N-(8-methyl-2-phenylimidazo[1,2-a]pyrazin-3-yl)-2-(10H-phenoxazin-10-yl)acetamide | C27 H21 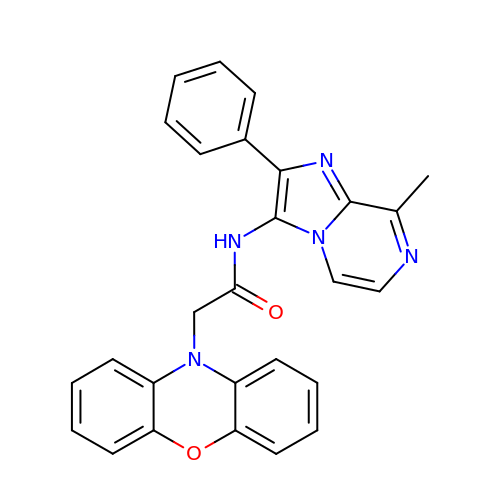N5 O2 | YQDHGEPNDQLBRG-UHFFFAOYSA-N> PVPTSGPSRKH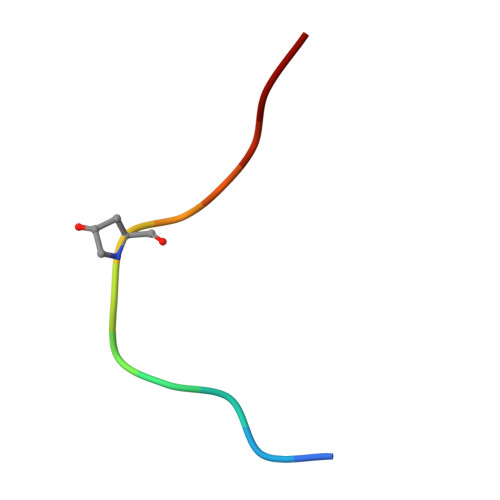N> SKPLLPIANPTVLRPANTFAITDTNDMSHSLALSNDTNVPFVKALDGSGLDEMSFDYLKKIPQFIQSKFFTT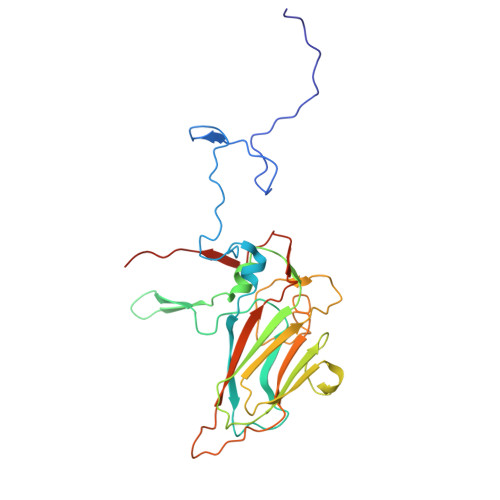TTKPQEVLFQTKVMPHYFVPGGDVTVAMDKDITRTIWQPSHLAYITSMFKYWTGSLVYTFKFVKTDYHSGRVEVSFHPFSDYTTGTYSDYTYRIIVDLREKSEFSVTIPFISPVPYKRISRPDWDKPYSKYAHASTGTLVLKALTSLKATNTVVSNSVEILIEVNAGDDFNVIAPIENIFFPFSLSPGRKGMVAQ>[2x]MSLRIGVIGTGAIGKEHINRITNKLSGAEIVAVTDVNQEAAQKVVEQYQLNATVYPNDDSLLADENVDAVLVTSWGPAHESSVLKAIKAQKYVFCEKPLATTAEGCMRIVEEEIKVGKRLVQVGFMRRYDSGYVQLKEALDNHVIGEPLMIHCAHRNPTVGDNYTTDM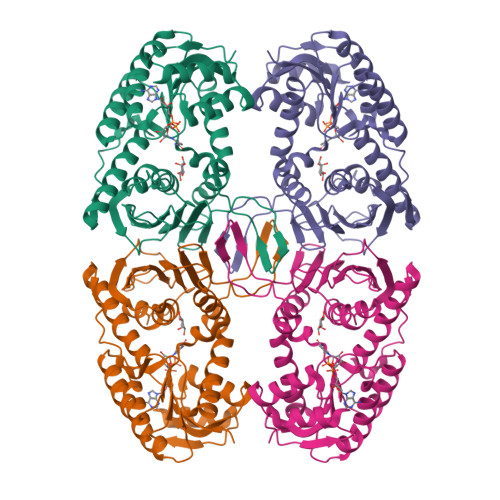AVVDTLVHEIDVLHWLVNDDYESVQVIYPKKSKNALPHLKDPQIVVIETKGGIVINAEIYVNCKYGYDIQCEIVGEDGIIKLPEPSSISLRKEGRFSTDILMDWQRRFVAAYDVEIQDFIDSIQKKGEVSGPTAWDGYIAAVTTDACVKAQESGQKEKVELKEKPEFYQSFTTVQN>[2x]GGCUCG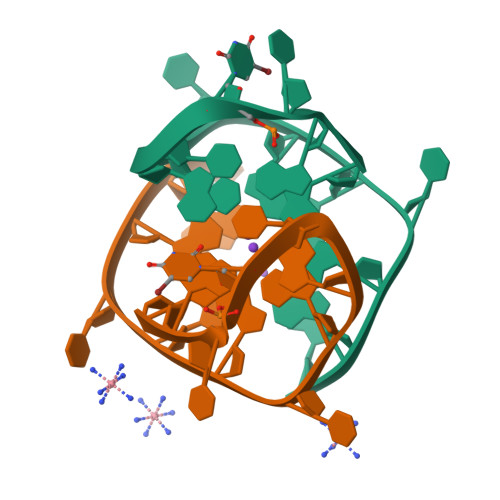GCGGCGGA> MSHHHHHHSGSGSGEKEEAEEVVKEALKELKKLFEEQKKVNEEAAKELEETAKDEKVLLAARFAVEASRIANKASFDLSKFAADAAAAAVEAGADIERVKEVLEKAIEAQKEAAKFSKKVLEEAAAAAALAERGEITEEDVARFVVELALELLKALFEMQRFVNELAAELLEVVAKDEKVLLAARFAVEASKIANEASFELSRFAAEAAAAAVEAGADIERVAEVLIKAIEAQAEAAKFSAEVLLKAAAAAALAERGEITEEDVARFVVELALELLRALFEMQRFVNELAAELLEVVAKDEKVLLAARFAVEASEIANKASFDLSKFAADAARAAVEAGADIERVAEVLIEAIKAQAEAAKFSAEVLLKAAAAAALAERGEITEKDVARFVVELALELLEALFEMQRFVNELAAALLEVVAKDEEVLEKARKAVEDSKRENEASFEESRKAAEAAAAAVEAGADIDEVAKELIEAIKEQAEAAKESAKKLLEAAAEAALAERGEIT

Here we describe extendable linear, curved and angled protein building blocks, as well as inter-block interactions, that conform to specified geometric standards; assemblies designed using these blocks inherit their extendability and regular interaction surfaces, enabling them to be expanded or contracted by varying the number of modules, and reinforced with secondary struts. We construct twistless helix repeat (THR) protein blocks from identical straight α-helices (typically 2–4 helices in each unit); the length of the blocks can be varied simply by varying the number of repeat units. Restricting helical geometry to ideal straight helices with zero helical twist in principle considerably limits what types of structure could be built, but this is more than compensated by the great simplification of downstream material design, as illustrated below. Using X-ray crystallography and electron microscopy, we validate nanomaterial designs ranging from simple polygonal and circular oligomers that can be concentrically nested, up to large polyhedral nanocages and unbounded straight ‘train track’ assemblies with reconfigurable sizes and geometries that can be readily blueprinted.

To generate straight, linear THRs, we set Δθ to zero. This results in perfectly straight repeat proteins in which each repeat unit is translated but not rotated relative to the previous unit. We tested 33 linear THRs (with Δh = 0) with helices either about 20 or about 40 residues in height; 23 of 33 tested designs were solubly expressed, and 13 of 19 designs analysed by SEC were primarily monomeric as designed. Structural characterization of the linear building blocks by X-ray crystallography individually and/or cryogenic EM (cryo-EM) in the context of assemblies (see below) revealed that both the detailed internal structures and the overall straight linear geometry were successfully achieved.> MAAVAVAVREDSGSGMKAELPPGPGAVGREMTKEEKLQLRKEKKQQKKKRKEEKGAEPETGSAVSAAQCQVGPTRELPESGIQLGTPREKVPAGRSKAELRAERRAKQEAERALKQARKGEQGGPPPKASPSTAGETPSGVKRLPEYPQVDDLLLRRLVKKPERQQVPTRKDYGSKVSLFSHLPQYSRQNSLTQFMSIPSSVIHPAMVRLGLQYSQGLVSGSNARCIALLRALQQVIQDYTTPPNEELSRDLVNKLKPYMSFLTQCRPLSASMHNAIKFLNKEITSVGSSKREEE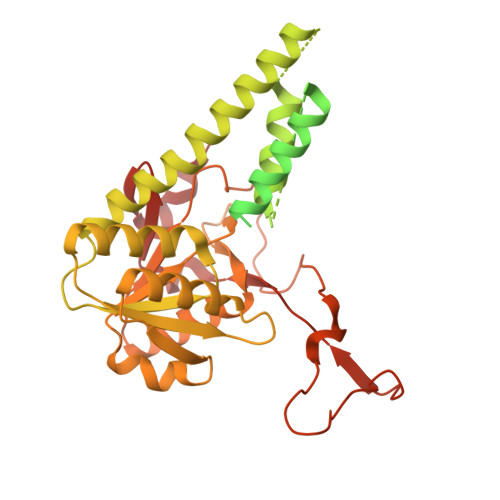AKSELRAAIDRYVQEKIVLAAQAISRFAYQKISNGDVILVYGCSSLVSRILQEAWTEGRRFRVVVVDSRPWLEGRHTLRSLVHAGVPASYLLIPAASYVLPEVSKVLLGAHALLANGSVMSRVGTAQLALVARAHNVPVLVCCETYKFCERVQTDAFVSNELDDPDDLQCKRGEHVALANWQNHASLRLLNLVYDVTPPELVDLVITELGMIPCSSVPVVARVKSSDQ> MRKYTFKTQRPKIVVIGGGTGLPVVLNGLRKQAVDITAVVTVADDGGSSGIIRNYVNVVPPGDIRNVMVALSSWPDLYKDIFQYRFQGDDQFFAGHAIGNLIIAALTEMKSGVFDAVQELSNMMQVDGHVYPAANEALTLHGKFSDGTELVGEAEITAAHK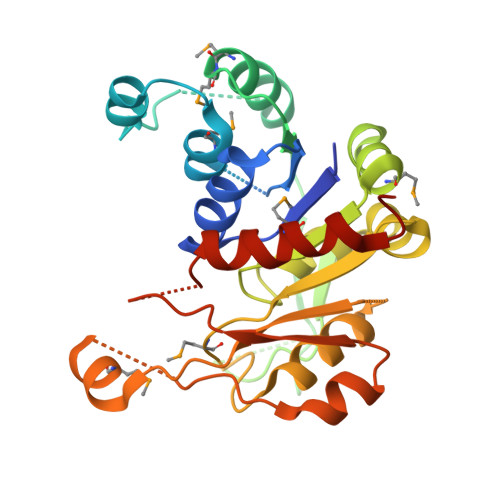SLERVWVTDKNGKEPQAVQPVIDAIMAADQIVLGPGSLFTSILPNLTIGNIGRAVCESDAEVVYICNIMTQKGETDNFSDADHVRVLNRHLGQNFINTVLVNTEKVPEDYMDFHKFNEVSKQVSHDFRGLREQNCRVISSNFLKLRDNGAFHDGDQVVAELMNLVGHSDVFRLEHHHHHH> MEPNEGVQLFSAFPPPPPYYKLFTRENIEKVISNMEKEAKHEDDANTLQPKTEEEIESLAKLFKKPSCLTSGTYQMFGDTWRLDEAIPSLKEFGIPELYKDIKDGEDEIEVVEYDPKSNAIVGTSFTRVHDYDKNSPIENEKI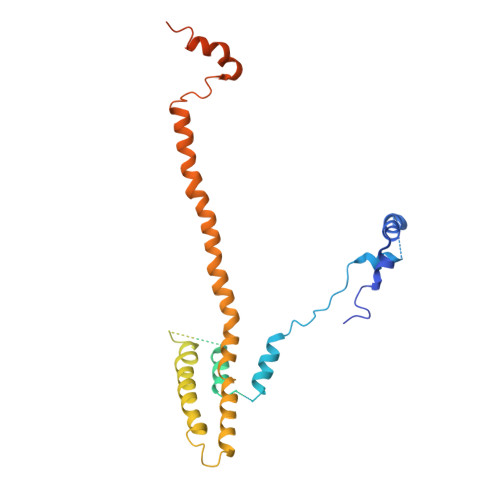LEDDQHTAMKEKDNESDKTMKDVEEKTEPSLKKEEEDIQMKEPLDSQDTGAVSASSVNEGFRADQKSKDGETSDLIKIPRRAYELRFLSRSLMLNFLELLGIMAKAPEQFPSKVENIRVLLLNLHHLINDYRPHQSRESLIMLLEKQLKHEESQVELLRTHNRQMTETLEKYKSLDFNMEKEGDVIQQLKSSIKKPLSGAEDEQKSRSMFSKNDEKLKKSLELMEDVIKRDLS>MEKVAFIGLGAMGYPMAGHLARRFPTLVWNRTFEKALRHQEEFGSEAVPLERVAEARVIFTC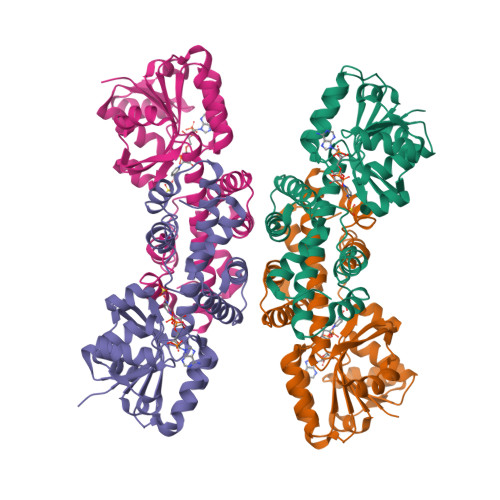LPTTREVYEVAEALYPYLREGTYWVDATSGEPEASRRLAERLREKGVTYLDAPVSGGTSGAEAGTLTVMLGGPEEAVERVRPFLAYAKKVVHVGPVGAGHAVKAINNALLAVNLWAAGEGLLALVKQGVSAEKALEVINASSGRSNATENLIPQRVLTRAFPKTFALGLLVKDLGIAMGVLDGEKAPSPLLRLAREVYEMAKRELGPDADHVEALRLLERWGGVEIR[4x]> RPESELIRQSWRVVSRSPLEHGTVLFARLFALEPSLLPLFQYNGRQFSSPEDSLSSPEFLDH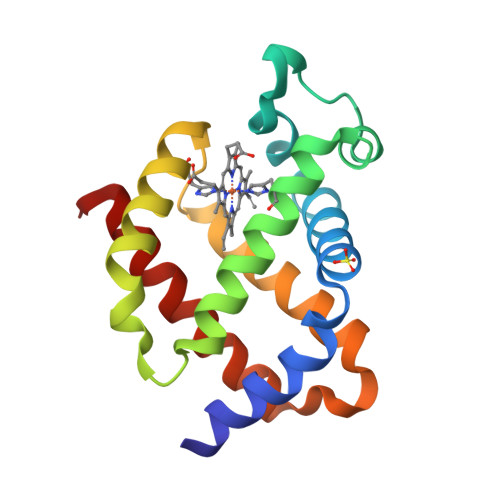IRKVMLVIDAAVTNVEDLSSLEEYLTSLGRKHRAVGFRLSSFSTVGESLLYMLEKSLGPDFTPATRTAWSRLYGAVVQAMSRGWDG> STMDWEVERAELQARIAFLQGERKGQENLKKDLVRRIKMLEY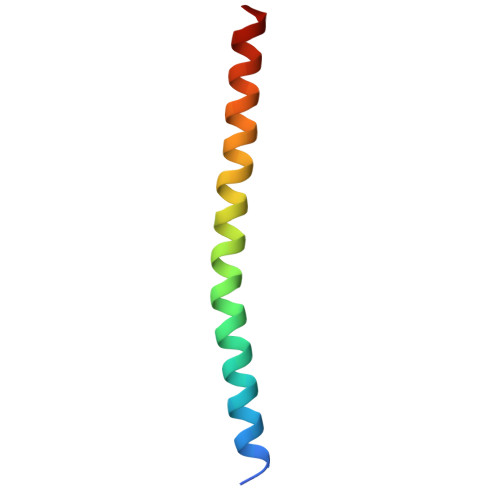ALKQERAK>[4x]MHHHHHHTSKIEQPRWASKDSAAGAASTPDEKIVLEFMDALTSNDAAKLIEYFAEDTMFQAMP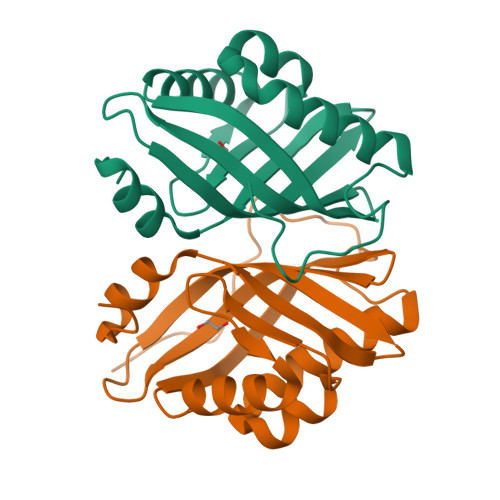LPPAYGRDAVEQTLAGLFTVMSFDAVETFHIGSSNGLVYTERVDVLRALPTGKSYNVSVLGVFQLTEGKITGWRDYFDLREFEEAVDLPLRG(2R,4aS,6aS,12bR,14aS,14bR)-10-hydroxy-2,4a,6a,9,12b,14a-hexamethyl-11-oxo-1,2,3,4,4a,5,6,6a,11,12b,13,14,14a,14b-tetradecahydropicene-2-carboxylic 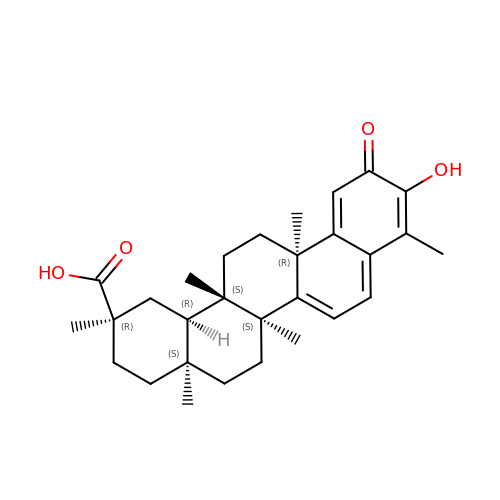acid | C29 H38 O4 | KQJSQWZMSAGSHN-JJWQIEBTSA-N>[2x]ASMTGGQQMGRGSSLTACPEESPLLVGPMLIEFNIPVDLKLVEQQNPKVKLGGRYTPMDCISPHKVAIIIPFRNRQ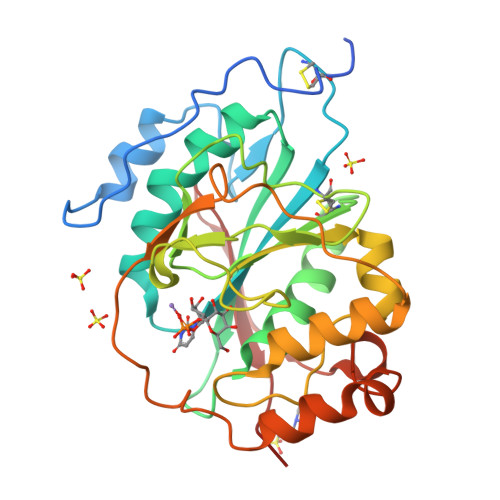EHLKYWLYYLHPILQRQQLDYGIYVINQAGESMFNRAKLLNVGFKEALKDYDYNCFVFSDVDLIPMNDHNTYRCFSQPRHISVAMDKFGFSLPYVQYFGGVSALSKQQFLSINGFPNNYWGWGGEDDDIYNRLAFRGMSVSRPNAVIGKTRHIRHSRDKKNEPNPQRFDRIAHTKETMLSDGLNSLTYMVLEVQRYPLYTKITVDIGTPS~{N}2-methyl-~{N}4-[(1~{S},2~{S})-2-methylcyclopropyl]-6-(phenylmethyl)pyridine-2,4-dicarboxamide 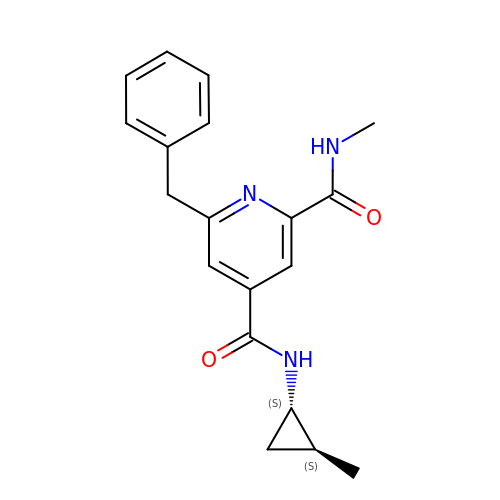| C19 H21 N3 O2 | QEPZFLZVHFIDCF-LRDDRELGSA-N> MDVYAQEKQDFVQHFSQIVRVLTEDEMGHPEIGDAIARLKEVLEYNAIGGKYNRGLTVVVAFRELVEPRKQDADSLQRAWTVGWCVELLQ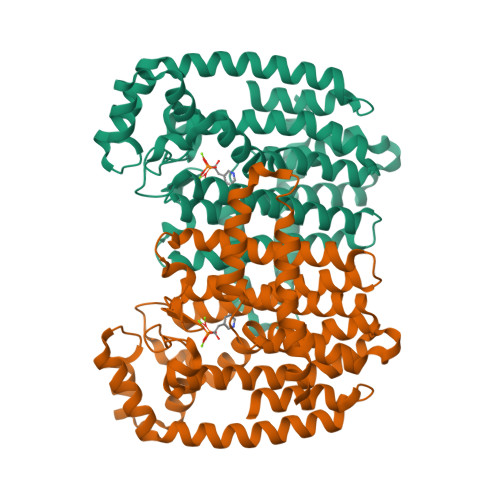AFFLVADDIMDSSLTRRGQICWYQKPGVGLDAINDANLLEACIYRLLKLYCREQPYYLNLIELFLQSSYQTEIGQTLDLLTAPQGNVDLVRFTEKRYKSIVKYKTAFYSFYLPIAAAMYMAGIDGEKEHANAKKILLEMGEFFQIQDDYLDLFGDPSVTGKIGTDIQDNKCSWLVVQCLQRATPEQYQILKENYGQKEAEKVARVKALYEELDLPAVFLQYEEDSYSHIMALIEQYAAPLPPAVFLGLARKIYKRRKLEHHHHHH>MHHHHHHGSGMAGLLKESMRIKMYMEGTVNGHYFKCEGEGDGNPFAGTQSMRIHVTEGAPLPFAFDILAPCCEYGSKTFVHHTAEIPDFFKQSFPEGFTWERTTTYEDGGILTAHQDTSLEGNCLIYKVKVHGTNFPADGPVMKNKSGGWEPSTEVVYP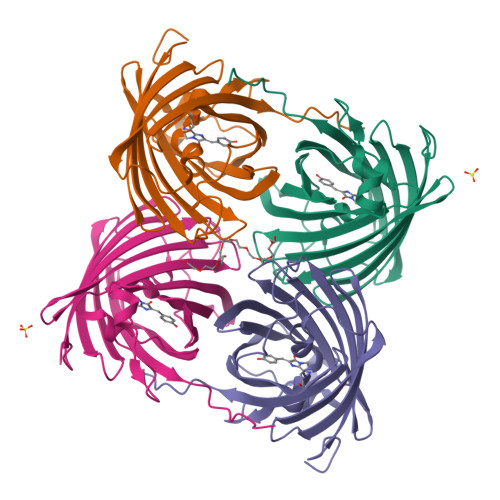ENGVLCGRNVMALKVGDRHLICHHYTSYRSKKAVRALTMPGFHFTDYRLQMLRKKKDEYFELYEASVARYSDLPEKAN[4x]> MGVFTFQDEYTSTIAPAKLYKALVTDADIIIPKAVETIQSVEIVEGNGGPGTIKKLTFIEGGESKYVLHKIEAIDEANL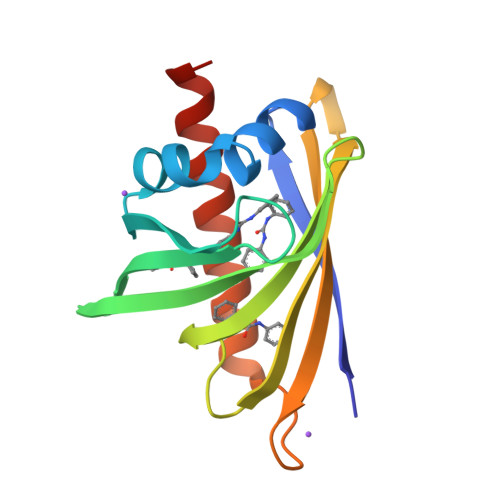GYNYSIVGGVGLPDTIEKISFETKLVEGANGGSIGKVTIKIETKGDAQPNEEEGKAAKARGDAFFKAIESYLSAHPDYN>[2x]VAFGADAAKTTQEKFDALKEAGVFSGYP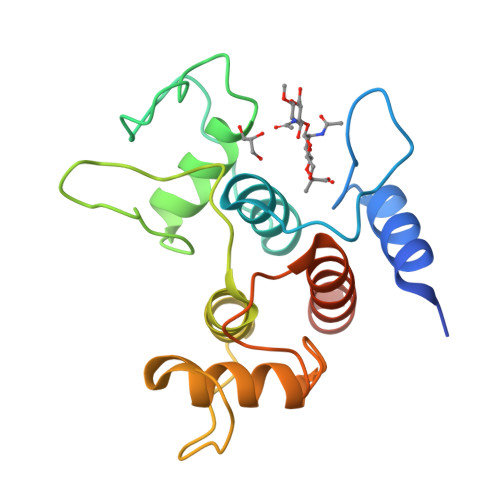GTTDAKLGQDMTRAEFAKVLVKLFGLKEIHGQYSYKDKNYDAKNWAAPFIEAVTAEGLMQAKDLTKKIFDFNGKITVEEASKTLVTALKLEPVKDAQNKATDWAKGYFEAAVNAGLFSKDANPKANATRAQLVEAAFAADEMSKGSGSHHHHHH> MSITLRTYIFLDALQPQLATFIGKTARGFLPVPGQASLWVEIA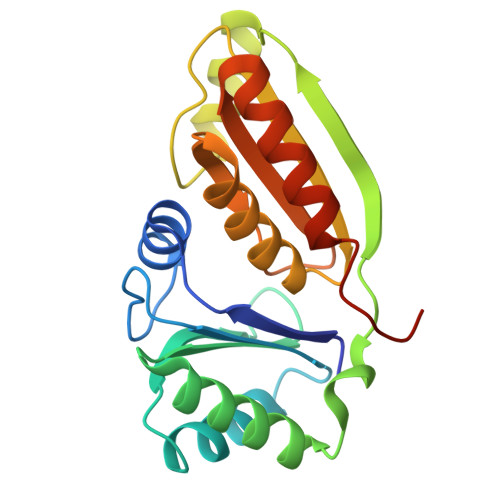PGIAINRVTDAALKATKVQPAVQVVERAYGLLEVHHFDQGEVLAAGSTILDKLEVREEGRLKPQVMTHQIIRAVEAYQTQIINRNSQGMMILPGESLFILETQPAGYAVLAANEAEKAANVHLVNVTPYGAFGRLYLAGSEAEIDAAAEAAEAAIRSVSGVAQESFRDR> MGSSHHHHHHSSGRENLYFQGSPVEKYNFKAEVNKVMDIIVNSLYTDKDVFLRELISNASDACDKKRIILENNKLIKDAEVVTNEEIKNETEKEKTENVNESTDKKENVEEEKNDIKKLIIKIKPDKEKKTLTITDNGIGMDKSELINNLGTIAQSGTA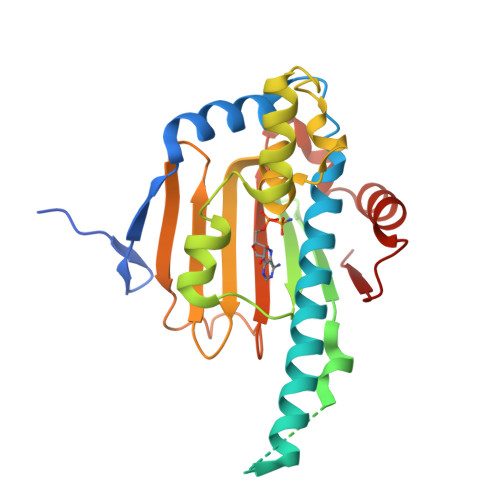KFLKQIEEGKADSNLIGQFGVGFYSSFLVSNRVEVYTKKEDQIYRWSSDLKGSFSVNEIKKYDQEYDDIKGSGTKIILHLKEECDEYLEDYKLKELIKKYSEFIKFPIEIWSE> LIKGPWTKEEDQRLIKLVQKYGPKRWS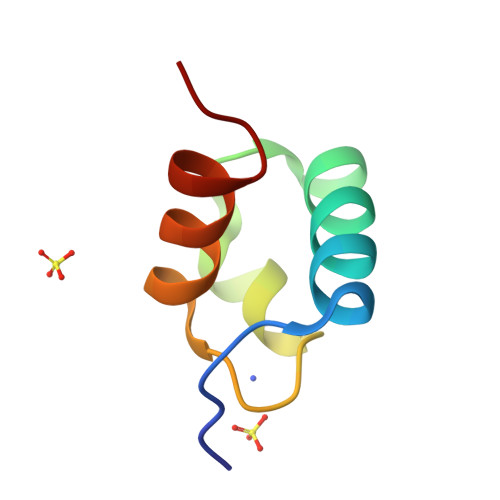VIAKHLKGRIGKQCRERWHNHLNPE> GSHMDYNKRSSVSTVPNAAPIRVGFVGLNAAKGWAIKTHYPAILQLSSQFQITALYSPKIETSIATIQRLKLSNATAFPTLESFASSSTIDMIVIAIQVASHYEVVMPLLEFSKNNPNLKYLFVEWALACSLDQAESIYKAAAERGVQTIISLQGRKSPYILRAKELISQGYIGDINSIEIAGNGGWYGYERPVKSPKYIYEIGNGVDLVTTTFGHTIDILQ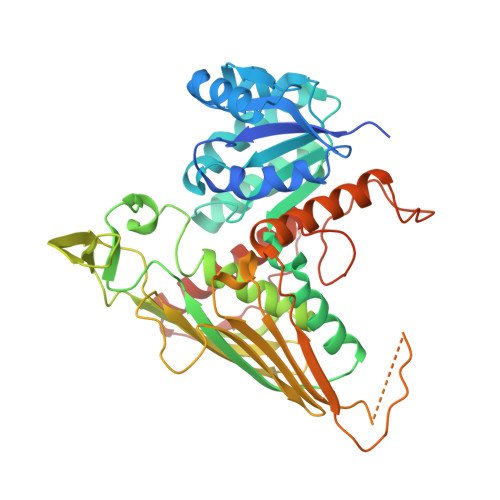YMTSSYFSRINAMVFNNIPEQELIDERGNRLGQRVPKTVPDHLLFQGTLLNGNVPVSCSFKGGKPTKKFTKNLVIDIHGTKGDLKLEGDAGFAEISNLVLYYSGTRANDFPLANGQQAPLDPGYDAGKEIMEVYHLRNYNAIVGNIHRLYQSISDFHFNTKKIPELPSQFVMQGFDFEGFPTLMDALILHRLIESVYKSNMMGSTLNVSNISHYSL> MPKRTDIKSILILGAGPIVIGQACEFDYSGAQACKALREEGYRVILVNSNPATIMTDPEMADATYIEPIHWEVVRKIIEKERPDAVLPTMGGQTALNCALELERQGVLEEFGVTMIGATADAIDKAEDRRRFDVAMKKIGLETARSGIAHTMEEALAVAADVGFPCIIRPSFTMGGSGGGIAYNREEFEEICARGLDLSPTKELLIDESLIGWKEYEMEVVRDKNDNCIIVCSIENFDAMGIHTGDSITVAPAQTLTDKEYQIMRNASMAVLREIGVETGGSNVQFAVNPKNGRLIVIEMNPRVSRSSALASKATGFPIAKVAAKLAVGYTLDELMNDITGGRTPASFEPSIDYVVTKIPRFNFEKFAGANDRLTTQMKSVGEVMAIGRTQQESLQKALRGLEVGATGFDPKVSLDDPEALTKIRRELKDAGADRIWYIADAFRAGLSVDGVFNLTNIDRWFLVQIEELVRLEEKVAEVGITGLNADFLRQLKRKGFADARLAKLAGVREAEIRKLRDQYDLHPVYKRVDTCAAEFATDTAYMYSTYEEECEANPSTDREKIMVLGGGPNRIGQGIEFDYCCVHASLALREDGYETIMVNCNPETVSTDYDTSDRLYFEPVTLEDVLEIVRIEKPKGVIVQYGGQTPLKLARALEAAGVPVIGTSPDAIDRAEDRERFQHAVERLKLKQPANATVTAIEMAVEKAKEIGYPLVVRPSYVLGGRAMEIVYDEADLRRYFQTAVSVSNDAPVLLDHFLDDAVEVDVDAICDGEMVLIGGIMEHIEQAGVHSGDSACSLPAYTLSQEIQDVMRQQVQKLAFELQVRGLMNVQFAVKNNEVYLIEVNPRAARTVPFVSKATGVPLAKVAARVMAGKSLAEQGVTKEVIPPYYSVKEVVLPFNKF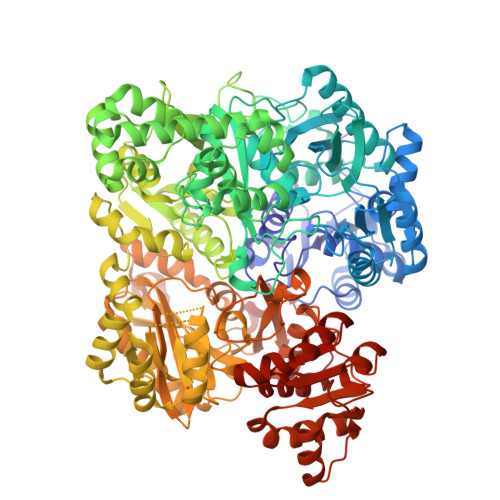PGVDPLLGPEMRSTGEVMGVGRTFAEAFAKAQLGSNSTMKKHGRALLSVREGDKERVVDLAAKLLKQGFELDATHGTAIVLGEAGINPRLVNKVHEGRPHIQDRIKNGEYTYIINTTSGRRAIEDSRVIRRSALQYKVHYDTTLNGGFATAMALNADATEKVISVQEMHAQIK The Notch signalling pathway is conserved across all metazoan species and plays key roles in many aspects of cell biology including cell‐fate determination, stem cell maintenance, immune system activation and angiogenesis in humans (Guruharsha et al, 2012; Bray, 2016). Aberrant Notch signalling results in a number of inherited and acquired disorders, including various cancers, and it is therefore a key target for therapeutic intervention (Hansson et al, 2004; Groth & Fortini, 2012). Both the Notch receptors and the ligands are single‐pass type I transmembrane proteins, and direct protein–protein contact between adjacent cells initiates an intracellular signalling pathway. All of the Notch ligands have a modular extracellular architecture consisting of an N‐terminal C2 domain (formerly known as the MNNL domain), a Delta/Serrate/Lag‐2 (DSL) domain, and either 16 (Jagged1/Jagged2), 8 (Delta‐like1/Delta‐like4) or 7 (Delta‐like3) EGF repeats. Binding of a Notch ligand to EGF11‐12 of a Notch receptor results in a series of proteolytic cleavages, with the final intra‐membrane cleavage by gamma secretase, causing the release of the intracellular domain of Notch (NICD) from the plasma membrane.

Here, we present the first structures of Jagged2 (N‐EGF2 and N‐EGF3), which has only 58% sequence identity with human Jagged1 (N‐EGF3), together with the longest known structure of a Delta‐like4 ligand (human Delta‐like4 N‐EGF3). Two crystal forms of Jagged2 (N‐EGF2) (green) and one crystal form of Jagged2 (N‐EGF3) (dark green) were solved, including a total of seven crystallographically independent copies of N‐EGF2, and 1 copy of N‐EGF3 (N.b. not all of EGF3 is visible in the electron density). All of these copies have been superposed on each other by alignment of the DSL domain, showing some flexibility in the hinge region between the C2 and DSL domains, and further flexibility in the hinge regions between the EGF domains. However, the angle between adjacent domains can vary subtly, resulting in the ligand structures appearing to fall into two groups, one group including Jagged1, Delta‐like1 and some structures of Jagged2, and the other including Delta‐like4, and some structures of Jagged2. The observation that Jagged2 is split across the two groups suggests that there is some flexibility between adjacent domains of the Notch ligands and that all may be able to adopt these different conformations. It is therefore likely that the conformation seen is determined by crystal packing. The Jagged1 and Jagged2 C2 domains bind calcium ions (shown in red), whereas Delta‐like4 and Delta‐like1 do not; the aspartates involved in calcium binding are not conserved in Delta‐like4 and Delta‐like1. The C2 loops are ordered upon calcium binding in both Jagged1 (Chillakuri et al, 2013) and Jagged2 and contain the amino acid ligands for calcium binding although the number of calcium ions bound differs.

>[6x]MGYFELQLSALRNVNGELLSGACCDGDGRTTRAGGCGHDECDTYVRVCLKEYQAKVTPTGPCSYGHGATPVLGGNSFYLPPAGAAGDRARARARAGGDQDPGLVVIPFQFAWPRSFTLIVEAWDWDNDTTPNEELLIERVSHAGMINPEDRWKSLHFSGHVAHLELQIRVRCDENYYSATCNKFCRPRNDFFGHYTCDQYGNKACMDGWMGKECKEAVCKQGCNLLHGGCTVPGECRCSYGWQGRFCDECVPYPGCVHGSCVEPWQCNCETNWGGLLCDKDLNGSHHHHHHHH>[2x]DSIMKILLIGDSGVGKSCLLVRFVEDKFNPSFITTIGIDFKIKTVDINGKKVKLQIWDTAGQERFRTITTAYYRGAMGIILVYDITDERTFTNIKQW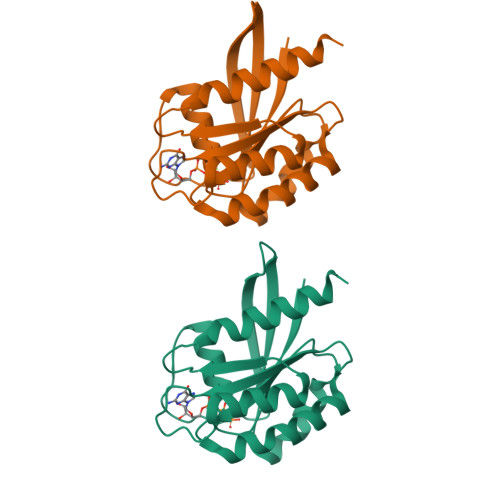FKTVNEHANDEAQLLLVGNKSDMETRVVTADQGEALAKELGIPFIESSAKNDDNVNEIFFTLAKLIQEKIDSN> MSEEEVSFSRDYFVEMDVRDEEAHELASDWFDEVVFTKKLVLED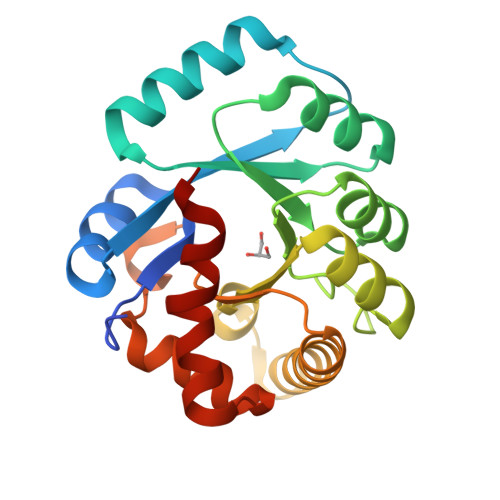PPDWGSLKEELKELRGKYGKVALLLVTRKPSLIREVKSRNLKALLYVQGGDMRINRMAIESGVDALISPWFGRKDPGFDHTLAGMAARRGVAIGFSLSPLLNANPYGRAQILRFMMKTWQLVKKYRVPRFITSSAESRWEVRGPRDLMSLGINIGMEIPEARASLNFYPRTIVWKL> GPGSDDEINAQSVWSEEISSNYPLCIKNLMEGLKKNHHLRYYGRQQLSLFLKGIGLSADEALK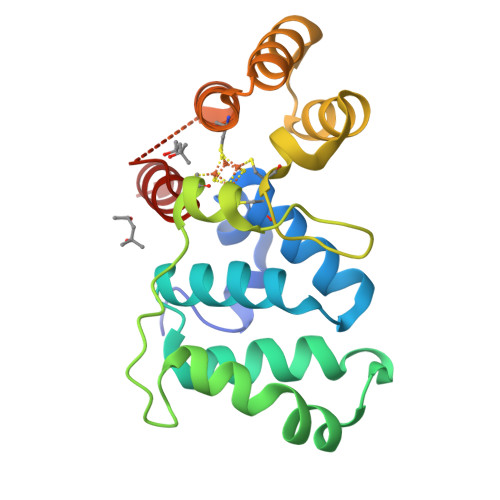FWSEAFTRNGNMTMEKFNKEYRLSFRHNYGLEGNRINYKPWDCHTILSKPRPGRGDYHGCPFRDWSHERLSAELRSMKLTQAQIISVLDSCQKGEYTIACTKVFEMTHNSASADLEIGEQTHIAHPNLYFERSRQLQK> MGSSHHHHHHSSENLYFQSHMTLPAFKAYDIRGRVPDELNEDLARRIGVALAAQLDQGPVVLGHDVRLASPALQEALSAGLRASGRDVIDIGLCGTEEVYFQTDYLKAAGGVMVTASHNPMDYNGMKLVREQARPISSDTGLFAIRDTVAADTAAPGEPTASEQSRTDKTAYLEHLLSYVDRSTLKPLKLVVNAGNGGAGLIVDLLAPHLPFEFVRVFHEPDGNFPNGIPNPLLPENRDATAKAVKDNGADFGIAWDGDFDRCFFFDHTGRFIEGYYLVGLLAQAILAKQPGGKVVHDPRLTWNTVEQVEEAGGIPVLCKSGHAFIKEKMRSENAVYGGEMSAHHYFREFAYADSGMIPWLLIAELVSQS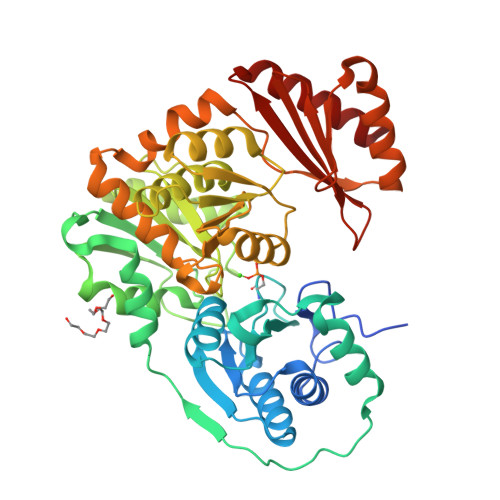GRSLADLVEARMQKFPCSGEINFKVADAKASVARVMEHYASLSPELDYTDGISADFGQWRFNLRSSNTEPLLRLNVETRGDAALLETRTQEISNLLRG A cleavage between the N-terminus of integrase (IN) and the C-terminus of the RNase H domain of RT produces mature IN and PR-RT from the Pol polyprotein. The mature PR-RT has all of the enzymatic functions of PR and RT [reviewed in [15]]. The PR-RTs of FVs are monomeric in solution and the RT component is responsible for converting the (+) FV ssRNA genome into dsDNA for integration into the host chromosome. The arrangement of the subdomains of PFV RT is similar to that of the p51 subunit of HIV-1 RT while the PR structurally resembles a single subunit of the catalytically active HIV-1 PR dimer.

Two mutations, H507D and S584K, were made in the PR-RT. In addition, we also made the C280S mutation to improve the solution behavior of the protein akin to HIV-1 RT C280S, which is known to improve the behavior of purified HIV-1 RT (it is a coincidence that these two residues, which are located in different subdomains in the respective proteins, have the same amino acid number, 280; they are not positional equivalents). The PR-RT mutant C280S/H507D/S584K, designated CSH, gave a 4-fold increase in expression compared to the WT in bacterial strains. When compared to WT, the CSH mutant had similar RNase H activity and showed a modest reduction in the polymerase activity. The higher purity and greater yield of the CSH mutant of PFV PR-RT made it possible to use broad robotic crystallization screens, which resulted in the growth of crystals that diffracted to ~3 Å resolution. The structure of the WT PR-RT was initially solved by using the anomalous signal from the selenomethionine (SeMet)-substituted CSH mutant, and the model obtained was used as the search model for molecular replacement using the WT data. The same crystallization condition that yielded the crystals of the CSH mutant did not produce usable crystals of the WT protein; relatively fragile, but usable, crystals of WT protein could be produced by modifying the crystallization conditions. Both the CSH mutant and WT PFV PR-RT crystallize as monomers with one copy in the asymmetric unit in space group C2. Despite differences in the unit-cell parameters, particularly along the x-axis, the structures of CSH and WT PR-RTs are highly superimposable (RMSD = 0.785 Å). The connection subdomain is further tilted slightly towards the polymerase active site such that it sits almost parallel to the palm of the RT compared to its position in the p66 subunit of HIV-1 RT where the two subdomains are orthogonal. This compact fold allows helix L (K in HIV-1 RT) to pack against H, while helix O (L in HIV-1 RT) tilts towards the active site loop positioning T552 of PFV RT to form a hydrogen bond with Y314, and T556 with H236, while H507 forms a bifurcated hydrogen bond with S237 and N364. The H507D mutant employed in the SeMet protein also makes analogous contacts, and the SeMet PR-RT crystallizes much faster than WT.

> QLLQPLPAEIKGTKLLAHWASGATITCIPESFLEDEQPIKKTLIKTIHGEKQQNVYYVTFKVKGRKVEAEVIASPYEYILLSPTDVPWLTQQPLQLTILVPLQEYQEKILSKTALPEDQKQQLKTLFVKYDNLWQHWENQVGHRKIRPHNIATGDYPPRPQKQYPINPKAKPSIQIVIDDLLKQGVLTPQNSTMNTPVYPVPKPDGRWRMVLDYREVNKTIPLTAAQNQHSAGILATIVRQKYKTTLDLANGFWAHPITPESYWLTAFTWQGKQYSWTRLPQGFLNSPALFTADVVDLLKEIPNVQVYVDDIYLSHDDPKEHVQQLEKVFQILLQAGYVVSLKKSEIGQKTVEFLGFNITKEGRGLTDTFKTKLLNITPPKDLKQLQSILGLLNFARNFIPNFAELVQPLYNLIASAKGKYIEWSEENTKQLNMVIEALNTASNLEERLPEQRLVIKVNTSPSAGYVRYYNETGKKPIMYLNYVFSKAELKFSMLEKLLTTMDKALIKAMDLAMGQEILVYSPIVSMTKIQKTPLPERKALPIRWITWMTYLEDPRIQFHYDKTLPELKHIPDVYTSSQKPVKHPSQYEGVFYTDGSAIKSPDPTKSNNAGMGIVHATYKPEYQVLNQWSIPLGNHTAQMAEIAAVEFACKKALKIPGPVLVITDSFYVAESANKELPYWKSNGFVNNKKKPLKHISKWKSIAECLSMKPDITIQHEKGHQPTNTSIHTEGNALADKLATQGSYVVN> KENGKRTEVKIGAKTSVMKEKDGKLFTGKANKETNKVDGANATEDADEGKGLVTAKDVIDAVNKTGWRIKTTDANGQNGDFATVASGTNVTFASGNGTTATVTNGTDGITVKYDAK

In a subset of nontypeable strains, the major nonpilus adhesin is a protein called Hia. Hia contains two homologous binding domains, called HiaBD1 and HiaBD2, that interact with the same host cell receptor. In particular, the Hia passenger domain consists of repeats of structurally similar domains, including five structurally identical Trp-ring domains strung together by two IsNeck domains and two KG domains.

Thus, the Ile residue at position 324 in the nonconserved region of KG1 was mutated to Met, allowing production of selenomethionine-derivatized crystals usable for phasing by the multiwavelength anomalous dispersion (MAD) method. The crystal structure of Hia307–422 was determined to a resolution of 1.8 Å. The nonadhesive Hia307–422 fragment contains three distinct domains, including the last strand of the preceding W2 domain (βW25), a novel “KG1” domain, and the W3 domain. βW25 lies in the crystal packing interface between two Hia307–422 trimers and forms an anti-parallel β-sheet with the adjacent βW25 strand of a separate trimer. Although the conformation of βW25 observed in Hia307–422 might not accurately reflect the conformation it adopts in the W2 domain, it may be used to envisage the structural transition between Trp-ring domains via a KG connector domain. The structure of the KG1 domain appears to be related to the structure of the IsNeck domain, with the secondary structures positioned similarly relative to each other. However, it must be noted that the topologies of the IN and KG domains(i.e., the way the secondary structures are connected) are very different. The W3 domain in Hia307–422 is similar to the W1 domain in HiaBD2 and to the W5 domains in HiaBD1, with the same number of strands and the same angle of the strands relative to the axis of the trimer. While HiaBD1 has structural similarities with Hia307–422, αIN3 in HiaBD1 does not have a corresponding region in KG1 in Hia307–422, and αIN2 in HiaBD1 is oriented differently from αKG1 in Hia307–422. Thus, two important structural determinants of binding in the IN domain are either absent or misoriented in the KG domain, explaining why Hia307–422 is nonadhesive.>[2x]AKLTIESTPFN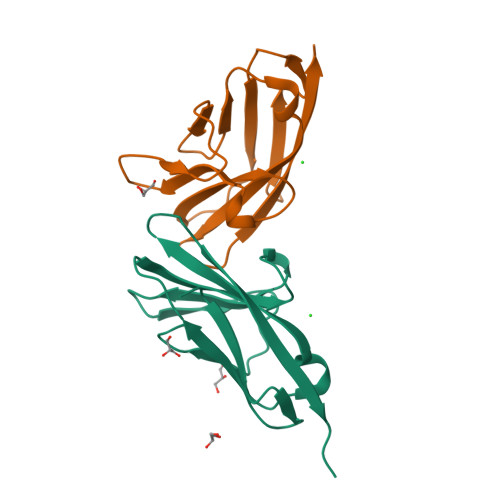VAEGKEVLLLVHNLPQHLFGYSWYKGERVDGNRQIIGYVIGTQQATPGPAYSGREIIYPNASLLIQNIIQNDAGFYTLHVIKSDLVNEEATGQFRVYPEL>MAEQTVEAPSVDARAWILMDYASGKVLAEGNADEKLDPASLTKIMTSYVVGQALKADKIKLTDMVTVGKDAWATGNPALRGSSVMFLKPGDQVSVADLNKGVIIQSGNDACIALADYVAGSQESFIGLMNGYAKKLGLTNTTFQTVHGLDAPGQFSTARDMALLGKALIHDVPEEYAIHKEKEFTFNKIRQPNRNRLLWSSNLNVDGMKTGTTAGAGYNLVASATQGDMRLISVVLGAKTDRIRFNESEKLLTWGFRFFETVTPIKPDATFVTQRVWFGDKSEVNLGAGEAGSVTIPRGQLKNLKASYTLTEPQLTAPLKKGQVVGTIDFQLNGKSIEQRPLIVMENVE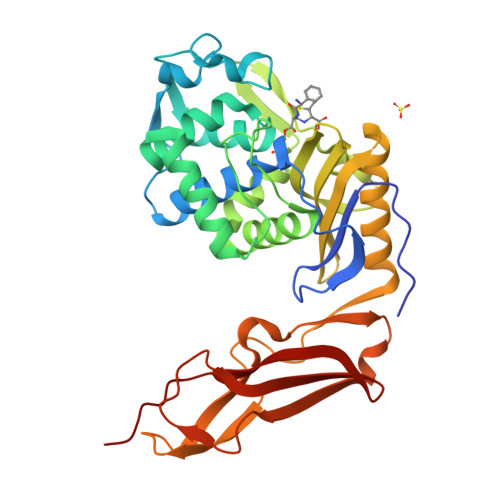EGG[4x]>[8x]MGSDKIHHHHHHMIVEERIYRIRGGKMQEYLKLVREEGIAIQAPILGNLIGYF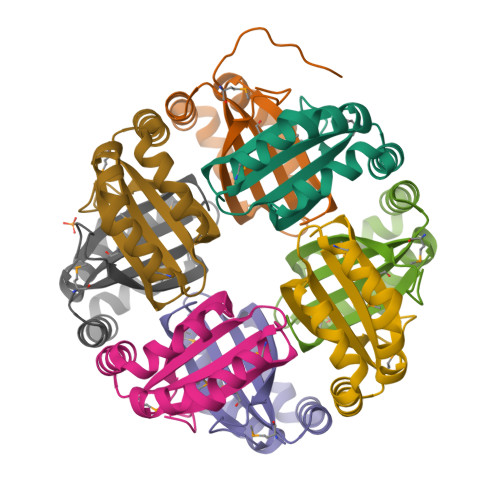VTDIGPLSQVIHMWGYASLDDRAERRGKLAEDQRWQAFIPRLSVLIESSENRILLPTDFSPLR> MTRIDAAPNPFHAAMQGRHDASANTSSGWLQGQRIAPAPTGISLADAAEELSLHMAQAAEEKHHSERKVTAERPMLWLDAAQLAELFSHTHDPDAQAKLEALTAELLRGRGAPMQLAAQAFPGVTQQYLALQHALQRGEHEDAAPHALEALRDALADLELAHGPEIRAGINTLPTAGAFARSADELAGFQHAYRDIALGQLS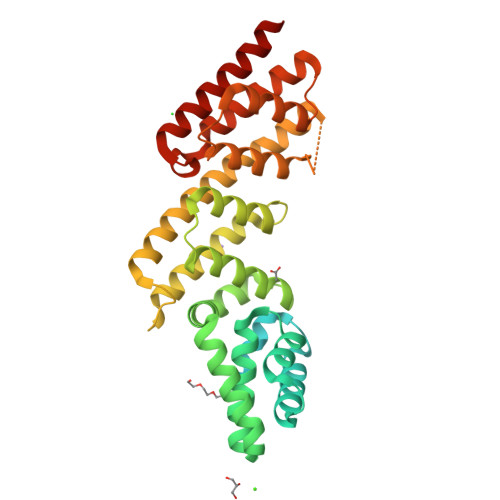LARTLDLVLERYGNDDIHGALGALIQALGHDLAAATPSTDGVRLQVLASDLYQVEVAATVLEECNALKQRLGNAGSQECADAQGLMRDLVGISEDKWIAPARFEKLAERHGANALSERIAFLGGVRQILKDLPTQIYADMDVRATVLAAAQDALDNAIAMENA> MFNRTTQLKSKHPCSVCTRRKVKCDRMIPCGNCRKRGQDSECMKSTKLITASSSKEYLPDLLLFWQNYEYWITNIGLYKTKQRDLTRTPANLDTDTEECMFWMNYLQKDQSFQLMNFAMENLGALYFGSIGDISELYLRVEQYWDRRADKNHSVDGKYWDALIWSVFTMCIYYMPVEKLAEIFSVYPLHEYLGSNKRLNWEDGMQLVMCQNFARCSLFQLKQCDFMAHPDIRLVQAYLILATTTFPYDEPLLANSLLTQCIHTFKNFHVDDFRPLLNDDPVESIAKVTLGRIFYRLCGCDYLQSGPRKPIALHTEVSSLLQHAAYLQDLPNVDVYREENSTEVLYWKIIS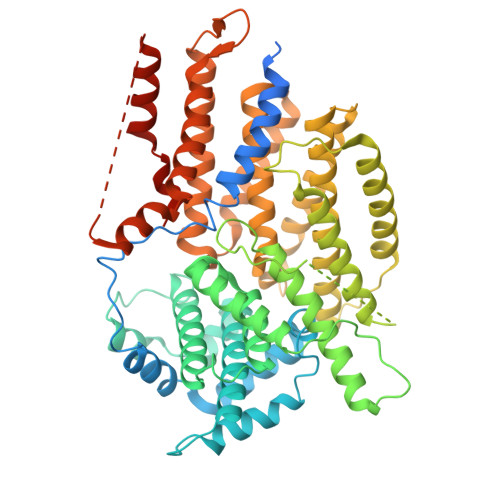LDRDLDQYLNKSSKPPLKTLDAIRRELDIFQYKVDSLEEDFRSNNSRFQKFIALFQISTVSWKLFKMYLIYYDTADSLLKVIHYSKVIISLIVNNFHAKSEFFNRHPMVMQTITRVVSFISFYQIFVESAAVKQLLVDLTELTANLPTIFGSKLDKLVYLTERLSKLKLLWDKVQLLDSGDSFYHPVFKILQNDIKIIELKNDEMFSLIKGLGSLVPLNKLRQESLLEEEDENNTEPSDFRTIVEEFQSEYNISDILSGSGGSGENLYFQ>[4x]MEFDENCSEIIKRNEWTNVQAKNINYLIIPIPYVIIHHTVSLECNSKDTCISNIENIRSYHMDTLNWHDIGYSFLIGGDGN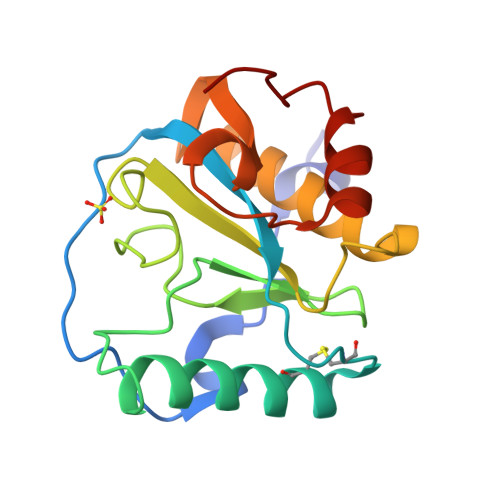IYEGCGWNHEGAHTYGYNKKSISIAFIGNFQNKSASNKMLNAAHKLILCGKSKGILREDVRVIGGKQVIATLSPGFELYKQIQNWPEWVSTP> EDAPVLSKAFVDRVNRLNRGIWKAKYDGVMQNITLREAKRLNGVIKKNNNASILPKRRFTEEEARAPLPSSFDSAEAWPNCPTIPQIA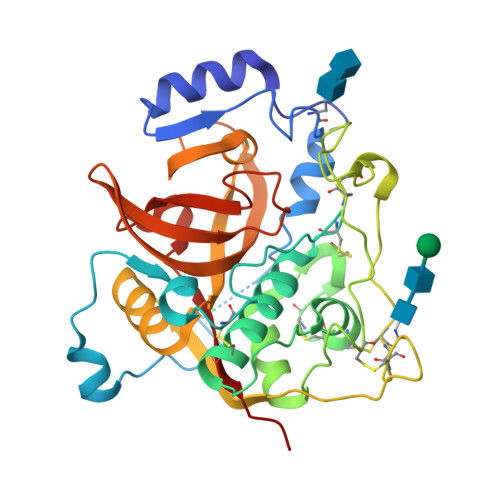DQSACGSCWAVAAASAMSDRFCTMGGVQDVHISAGDLLACCSDCGDGCNGGDPDRAWAYFSSTGLVSDYCQPYPFPHCSHHSKSKNGYPPCSQFNFDTPKCNCTCDDPTIPVVNYRSWTSYALQGEDDYMRELFFRGPFEVAFDVYEDFIAYNSGVYHHVCGQYLGGHAVRLVGWGTSNGVPYWKIANSWNTEWGMDGYFLIRRGSSECGIEDGGSAGIPLAPN> ANFENFIGATEGFSEIAYQFTSHILTLGYAVMLAGLLYFILTIKNVDKKFQMSNILSAVVMVSAFLLLYAQAQNWTSSFTFNEEVGRYFLDPSGDLFNNGYRYLNWLIDVPMLLFQILFVVSLTTSKFSSVRNQFWFSGAMMIITGYIGQFYEVSNLTAFLVWGAISSAFFFHILWVMKKVINEGKEGISPAGQKILSNIWILFLISWTLYPGAYLMPYLTGVDGFLYSEDGVMARQLVYTIADVSSKVIYGVLLGNLAITLSK

Here, we describe a multi-reservoir, high viscosity extruder as a step towards automation of sample delivery at XFELs. After commissioning the device with lysozyme crystals, we collected time-resolved data using crystals of a membrane-bound, light-driven sodium pump. Static data were also collected from the soluble protein tubulin that was soaked with a series of small molecule drugs. In two commissioning beamtimes at the SwissFEL Alvra endstation, we validated the general performance of the multi-reservoir extruder and determined 13 structures overall.

Second, we utilise the device in a time-resolved serial femtosecond crystallography (TR-SFX) experiment by collecting structural snapshots of the light-driven sodium pump Krokinobacter eikastus rhodopsin 2 (KR2). Xtrapol848 was used to calculate q-weighted difference maps Folight–Fodark and corresponding extrapolated maps from these data. These maps depicted the structural changes 1 μs after retinal photoactivation. C Difference electron density maps (FoLight–FoDark) shown at sigma level of 3.0 depicting the structural changes of and around the retinal 1 μs after photoactivation.>[2x]MLRIIDTETCGLQGGIVEIASVDVIDGKIVNPMSHLVRPDRPISPQAMAIHRITEAMVADKPWIEDVIPHYYGSEWYVAHNASFDRRVLPEMPGEWICTMKLARRLWPGIKYSNMALYKTRKLNVQTPPGLHHHRALYDCYITAALLIDIMNTSGWTAEQMADITGRLEHHHHHH

ExoX is one of several redundant exonucleases involved in the mismatch repair system, UV repair, homologous recombination and the stabilization of tandem repeats in E. coli. Like TREX1/2, ExoX contains only an exonuclease domain; however, it can act on both ssDNA and dsDNA in a distributive manner and digests only one or two nucleotides per reaction cycle. To elucidate the mechanism by which dsDNA is recognized and processed by single-domain DnaQ members, such as ExoX and TREX1/2, we determined the structures of ExoX in complex with three distinct dsDNA substrates: 3′ overhanging duplex DNA, a 12 bp blunt-ended dsDNA and 5′ overhanging partially mismatched duplex DNA, referred to here as complexes I, II and III, respectively. The crystal structures obtained revealed that ExoX interacts with dsDNA via two DNA-binding sites, one for the substrate strand and another for the complementary strand.

Our structure of the blunt-ended DNA complex is the first to show the specific interaction of a DnaQ member with a blunt-ended dsDNA. Similar to complex I, two ExoX monomers bind to the individual ends of one DNA molecule. First, in addition to the two residues that interacted with the complementary strand and were observed in the 3′ overhanging DNA complex (Lys101 and Arg104), an adjacent positively charged Arg87 residue was also involved in complementary strand binding via an interaction with the +2 and +3 nucleotides of the 5′ terminus. Second, the coordination of MeA in complexes I and II is different. Compared with the penta-coordination observed in complex I, MeA is tetra-coordinated in complex II, with one proposed water nucleophile missing, accompanied by a slight reorientation of the His134 side chain closer to the substrate phosphate. This difference may be attributed to the pH at which the crystals were grown (8.0 for complex I and 6.3 for complex II). Third, at both DNA ends (A and B) in complex II, a wedge composed of two key residues (Leu12 and Gln13) located in the loop between β1 and β2 (loop 1) was observed. Leu12 penetrates between the two terminal base pairs, while Gln13 is inserted halfway between the two terminal base pairs and forms an interaction with the second nucleotide of the 5′ terminus. The wedging of Leu12 and Gln13 results in a distortion of the first base pair and facilitates full insertion of the first substrate nucleotide into the active center. Therefore, the structure of complex II suggests that ExoX unwinds the first base pair of the blunt-ended dsDNA and feeds the 3′ end of the substrate strand into the active center.> MVMAPTLQ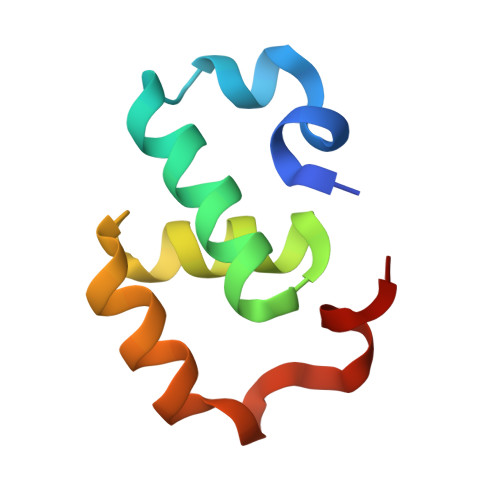LPPDVQSRLNPVQLELLNKLHLETKLNAEYTFMLAEQSNWNYEVAIKGFQSSMNGIPREAFVQF>MATITGAQIVARALKQQGVEHMFGIVGIPVIPIAAAAQREGIKFYGFHNEQSASYAAGAVGYLTGRPGVCLAVSGPGMIHGIAGLANAWSNNWPMILIGGANDSYQNGQGAFQEAPQIESARPYVKYAARPDSIARLPFYVEQAVRTTIYGRPGAAYLDLPGDIISGSVEEAEVTYPGRCPEPPRTLAPEENIKAALAALKTAERPLVIVGKGAAYSRAEDEVRKFVETTGLPYLASPMGKGVIPDDHPQSIAAARSFALQNTDLVVLMGARMNWMMHFGQPPRWNEKVRVIQMDISAEEIGTNVPTEVALVGDAKAITAQLNAELEKNPWSYPSETTWWTGLQSKIAANAATVEPMFNDDSVPMGYYRVLRDIRDLIPKDAIISNEGASTMDIGRTVLPNFFARTRLDAATFGTMGVGAGQAIAAASVHPDRKIICVQGDSAFGFGGMEVETAARYGLNITFVIINNNGIGGGPDELDPAHIPPGAYTPQAHYEKMADVYGGKGYFVTTPDQLKPVLEEAMAQPKPAIVNIMISNKSGRKPQEFGWLTR[2x]

One such enzyme is 2-hydroxyacyl-CoA lyase/synthase (HACL/S), which catalyzes the reversible cleavage of 2-hydroxyacyl-CoA (2hcCoA) into formyl-CoA (fCoA) and an aldehyde or ketone. Originally identified in the mammalian α-oxidation pathway of 3-methyl-branched fatty acids, HACL/S has demonstrated remarkable catalytic reversibility, as it is capable of condensing fCoA with various substrates covering a wide range of aldehydes and ketones with different carbon chain lengths. All the enzymes are tetramers, specifically dimers of dimers (α2), where α2 dimer represents a catalytical unit. The three domains have specific functions: the N-terminal domain binds the pyrimidine of ThDP (PYR), the middle domain has a regulatory function (R) and binds ADP, and the C-terminal domain binds the pyrophosphoryl group (PP) of ThDP.

TbHACL/S was co-crystallized in the presence of fCoA and hCoA. On the other hand, the asymmetric units of CoA compound-TbHACL/S complex contain only two slightly different monomers (protein chains A and B), each protomer from two separate catalytic pairs (AA’ and BB’, a prime indicates symmetry related partner), which means each catalytic dimer is formed by the structurally identical monomers. However, in the tetramer, the two dimers are slightly different, but contain identical catalytic sites. Several residues engage in close contacts with acyl-CoA (R545, K546, Q548, and W552 in ApbHACL/S and R540, K541, Q543 and W547 in TbHACL/S) through electrostatic, hydrogen bonds and van der Waals interactions. The C-terminal covering regions are coming from the second protomer. These contacts seem stabilizing and augmenting cofactor interactions with the active site, likely extending the “on” state of the acyl-CoA. ApbHACL/S has stronger activity on C2 (acetaldehyde) compared to C1 (formaldehyde) and C3 (propionaldehyde) substrates, while TbHACL/S discriminates less harshly between substrate chain length. Structures of both TbHACL/S and ApbHACL/S with and without acyl-CoA indicate that there is no notable difference in main chains and side chains except for the well-ordered C-terminal regions.>[2x]ADPCDLPQTHSLGSRRTLMLLAQMRRISLFSCLKDRHDFGFPQEEFGNQFQKAETIPVLAAMIAQIFNLFSTKDSSAAWDET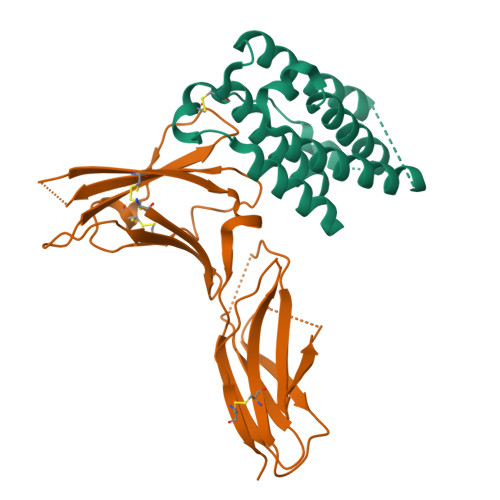LLDKFYTELYQQLNDLEACVIQGVGVTETPLMKEDSILAVRKYFQRITLYLKEKKYSPCAWEVVRAEIMRSFSLSTNLQESLRSKE;>[2x]ADPESCTFKISLRNFRSILSWELKNHSIVPTHYTLLYTIMSKPEDLKVVKNCANTTRSFCDLTDEWRSTHEAYVTVLEGFSGNTTLFSCSHNFWLAIDMSFEPPEFEIVGFTNHINVMVKFPSIVEEELQFDLSLVIEEQSEGIVKKHKPEIKGNMSGNFTYIIDKLIPNTNYCVSVYLEHSDEQAVIKSPLKCTLLPP>[41x]MRINHNIAALNTLNRLSSNNSASQKNMEKLSSGLRINRAGDDAAGLAISEKMRGQIRGLEMASKNSQDGISLIQTAEGALTETHAILQRVRELVVQAGNTGTQDKATDLQSIQDEISALTDEIDGISNRTEFNGKKLLDGTYKVDTATPANQKNLVFQIGANATQQISVNIEDMGADALGIKEADGSIAALHSVNDLDVTKFADNAADCADIGFDAQLKVVDEAINQVSSQRAKLGAVQNRLEHTINNLSASGENLTAAESRIRDVDMAKEMSEFTKNNILSQAPQAMLAQANQQPQNVLQLLR

There are three parts to the flagellar structure: the trans-membrane basal body that functions as the motor, the connecting rod and hook, and the flagellar filament that acts like a helical propeller. Our current understanding of supercoiling in bacterial flagellar filaments, referred to as polymorphic switching, is based upon the notion that protofilaments within the flagellar filament can exist in two discrete states, that differ slightly in length. The “short” state results from a protofilament having a right-handed inclination (the R-state), while the “long” state results from a protofilament having a left-handed inclination (the L-state). To reconstruct filaments at high resolution, all protofilaments must be “locked” into the same state, either L- or R-type, producing straightened filaments that lead to non-motile bacteria.

While the three L-type mutants (E115G, S285P, and S17P) have a left-handed 11-start helix, the four R-type mutants (N226Y, A233V, H84R and A39VN133H) have a right-handed 11-start helix, and the designations L and R correspond to the hand of these 11-start helices. The L-type 11-start helices are tilted left by ~ 1.7° and the R-type 11-start helices are tilted right by ~ 3.9°. Strikingly, we found those sites are not necessarily conserved among different species or participate in unique inter-subunit interactions. These include three straight mutations outside of the D1 helices: S17P, S285P (both within D0) and the double mutant A39V/N133H (within the loop region). We also detected two mutations, S17P and S285P, located in the middle of the small coiled-coil D0 domain. These two residues are not conserved in other species, and proline is not found at this position in any wildtype species. Therefore, mutation S17P or S285P in B. subtilis forces a local bend of ~ 30° in the helix axis, and this conformational change makes the D0 coiled-coil adopt an L-type form more easily. Here our high-resolution reconstructions expand our knowledge and we can now observe how mutations in D0 can cause a switching of the flagellar structure.>AEPVYPDQLRLFSLGQGVCGDKYRPVNREEAQSVKSNIVGMMGQWQISGLANGWVIMGPGYNGEIKPGTASNTWCYPTNPVTGEIPTLSALDIPDGDEVDVQWRLVHDSANFIKPTSYLAHYLGYAWVGGNDSQYVGEDMDVTRDGDGWVIRGNNDGGCDGYRCGDKTAIKVSNFAYNLDPDSFKHGDVTQSDRQLVKTVVGWAVNDSDTPQSGYDVTLRYDTATNWSKTNTYGLSEKVTTKNKFKWPLVGETELSIEIAANQSWASQNGGSTTTSLSQSVRPTVPARSKIPVKIELYKADISYPYEFKADVSYDLTLSGFLRWGGNAWYTHPDNRPNWNHTFVIGPYKDKASSIRYQWDKRYIPGEVKWWDWNWTIQQNGLSTMQNNLARVLRPVRAGITGDFSAESQFAGNIEIGAPVPLAADSKVRRARSVDGAGQGLRLEIPLDAQELSGLGFNNVSLSVTPAANQ[2x]

Aerolysin is produced by the human pathogen Aeromonas hydrophila as an inactive precursor called proaerolysin. Conversion of proaerolysin to aerolysin involves proteolytic cleavage of a flexible 43-residue loop near the C-terminus. The protein is L-shaped, composed of a continuous globular N-terminal domain, Domain 1, and an elongated region consisting of three discontinuous structural domains. Domain 4 has no known function but contains the CTP, which is folded as 2 anti-parallel β-strands connected by a short α-helix.

Residue His-132 is required for heptamer formation. Our MD-based observations thus suggest that the CTP remains bound to aerolysin upon proteolytic activation of the protoxin.>[2x]GSKNLIGRHLRLGSVEEQPFMFFATEGCEGNDCWSGMVNDMVVKLSEDLGFTYEYIQPDDRKFGALNKTTNEWNGMIRDLLDDKTDMIAIDLSTNSARKSAIDYSFPFMDAGIKAVVKGEGTTLNQVLELLDQDKYKWGVIGSRHPETLLKTHRDSRYSRLV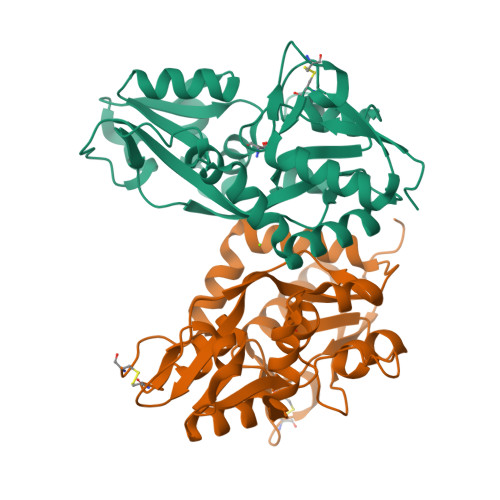DEGVELKDLNHAIETLRGGLFVFIDEGPVLAHNLISDCDVFSVGEEFQSFEYAFGLPKDSPYKSLIDSHLLKFREEGFIDILWEKWSSGNSVCS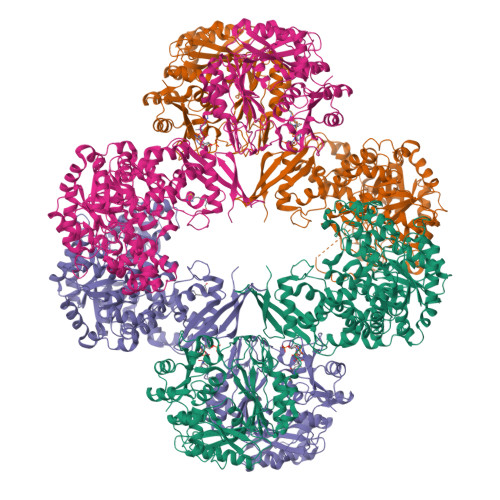>[4x]MKQIKKLLVANRGEIAIRIFRAAAELDISTVAIYSNEDKSSLHRYKADESYLVGSDLGPAESYLNIERIIDVAKQANVDAIHPGYGFLSENEQFARRCAEEGIKFIGPHLEHLDMFGDKVKARTTAIKADLPVIPGTDGPIKSYELAKEFAEEAGFPLMIKATSGGGGKGMRIVREESELEDAFHRAKSEAEKSFGNSEVYIERYIDNPKHIEVQVIGDEHGNIVHLFERDCSVQRRHQKVVEVAPSVGLSPTLRQRICDAAIQLMENIKYVNAGTVEFLVSGDEFFFIEVNPRVQVEHTITEMVTGIDIVKTQILVAAGADLFGEEINMPQQKDITTLGYAIQCRITTEDPLNDFMPDTGTIIAYRSSGGFGVRLDAGDGFQGAEISPYYDSLLVKLSTHAISFKQAEEKMVRSLREMRIRGVKTNIPFLINVMKNKKFTSGDYTTKFIEETPELFDIQPSLDRGTKTLEYIGNVTINGFPNVEKRPKPDYELASIPTVSSSKIASFSGTKQLLDEVGPKGVAEWVKKQDDVLLTDTTFRDAHQSLLATRVRTKDMINIASKTADVFKDGFSLEMWGGATFDVAYNFLKENPWERLERLRKAIPNVLFQMLLRASNAVGYKNYPDNVIHKFVQESAKAGIDVFRIFDSLNWVDQMKVANEAVQEAGKISEGTICYTGDILNPERSNIYTLEYYVKLAKELEREGFHILAIKDMAGLLKPKAAYELIGELKSAVDLPIHLHTHDTSGNGLLTYKQAIDAGVDIIDTAVASMSGLTSQPSANSLYYALNGFPRHLRTDIEGMESLSHYWSTVRTYYSDFESDIKSPNTEIYQHEMPGGQYSNLSQQAKSLGLGERFDEVKDMYRRVNFLFGDIVKVTPSSKVVGDMALYMVQNDLDEQSVITDGYKLDFPESVVSFFKGEIGQPVNGFNKDLQAVILKGQEALTARPGEYLEPVDFEKVRELLEEEQQGPVTEQDIISYVLYPKVYEQYIQTRNQYGNLSLLDTPTFFFGMRNGETVEIEIDKGKRLIIKLETISEPDENGNRTIYYAMNGQARRIYIKDENVHTNANVKPKADKSNPSHIGAQMPGSVTEVKVSVGETVKANQPLLITEAMKMETTIQAPFDGVIKQVTVNNGDTIATGDLLIEIEKATD>DTGERRCDPIRISMCQNLGYNVTKMPNLVGHELQTDAELQLTTFTPLIQYGCSSQLQFFLCSVYVPMCTEKINIPIGPCGGMCLSVKRRCEPVLKEFGFAWPESLNCSKFPPQNDHNHMCMEGPGDEEVPLPHKTPIQPGEGTLEVLFQ[4x]

Norrie Disease Protein (NDP) gene encodes Norrin, a secreted cystine-knot like growth factor, distinct from the lipid-modified Wnt. Unlike Wnts which have promiscuous interactions with Fz receptors, Norrin specifically binds to Fz4CRD, but not to the 14 other CRDs of Fz and secreted Frizzled-related protein (sFRP) family members. The Norrin mediated pathway maintains the blood-retina and blood-brain barriers and regulates angiogenesis in the cochlea and uterus as well as neuroprotective effects on retinal neurons. Our crystallographic and solution studies further reveal that dimeric Norrin forms a complex with two copies of monomeric Fz4CRD.

We determined two crystal structures of Fz4CRD. Similar to mouse Fz8CRD the Fz4CRD fold comprises four α helices stabilized by five disulphide bridges (Cys45–Cys106, Cys53–Cys99, Cys90–Cys128, Cys117–Cys158, Cys121–Cys145). The N-acetylglucosamines on two N-linked glycosylation sites at Asn59 and Asn144 are visible in the electron density map. Superposition of all Fz4CRD molecules in the asymmetric units from two crystal forms revealed a well-ordered protein fold. Structural comparison showed Fz4CRD closely resembles the CRDs of mouse Fz8 and secreted Frizzled-related protein 3 (sFRP3) with an average r.m.s. deviation of 1.2 Å over 115 equivalent Cα atoms and approximate sequence identity of 35%. Interestingly, we found that our Fz4CRD structures form the same dimeric assembly in two crystal lattices (r.m.s. deviation of 0.7 Å over 238 equivalent Cα atoms from two crystal forms). The dimer interface has an average 1330 Å2 buried surface area, in agreement with the characteristics of known protein–protein interfaces. However, this Fz4CRD dimer (front-to-front) is distinct from the previously reported crystal structure of mouse Fz8CRD dimer (back-to-back). Size-exclusion chromatography coupled to multi-angle light scattering (SEC-MALS) results showed Fz4CRD, Fz5CRD and Fz8CRD exist as monomers in solution at 50 μM concentration, in agreement with previously reported SEC studies of Fz8CRD and SEC-MALS analyses of MuSKCRD and SmoCRD. Taken together, our results suggest that the CRDs of Fz receptors exist as monomers and may not be involved in receptor dimerization; multiple GPCRs dimerize through their hepta-helical transmembrane domains.> EDPQGDAAQKTDTSHHDQDHPTFNKITPNLAEFAFSLYRQLAHQSNSTNIFFSPVSIAAAFAMLSLGAKGDTHDEILEGLNFNLTEIPEAQIHEGFQELLRTLNQPDSQLQLTTGNGLFLSEGLKLVDKFLEDVKKLYHSEAFTVNFGDTEEAKKQINDYVEKGTQGKIVDLVKELDRDTVFALVNYIFF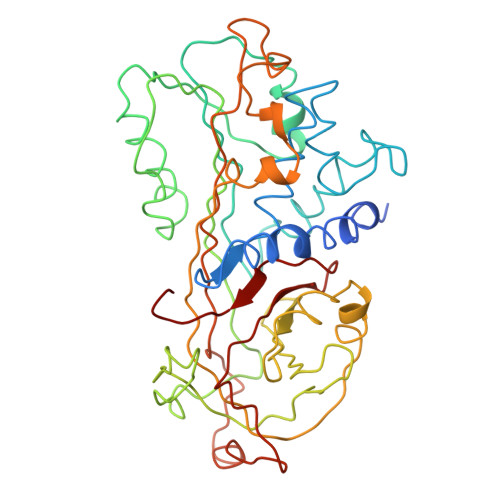KGKWERPFEVKDTEEEDFHVDQVTTVKVPMMKRLGMFNIQHCKKLSSWVLLMKYLGNATAIFFLPDEGKLQHLENELTHDIITKFLENEDRRSASLHLPKLSITGTYDLKSVLGQLGITKVFSNGADLSGVTEEAPLKLSKAVHKAVLTIDEKGTEAAGAMFLEAIPMSIPPEVKFNKPFVFLMIEQNTKSPLFMGKVVNPTQK(4-methylphenyl) hydrogen sulfate | 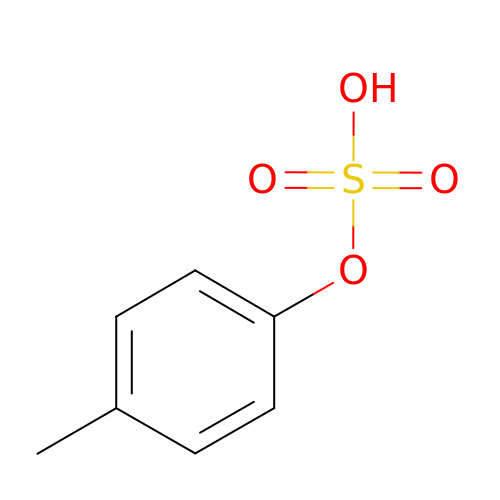C7 H8 O4 S | WGNAKZGUSRVWRH-UHFFFAOYSA-N In this study, we report the discovery and characterization of a new psychrophilic laccase, a multicopper oxidase (MCO), from the bacterium Oenococcus oeni. Laccases (benzenediol:oxygen oxidoreductase, p-diphenol oxidase EC 1.10.3.2) are blue multicopper oxidases (MCO), copper-containing enzymes that catalyse the oxidation of a substrate reducing molecular oxygen to water. Biochemical characterization of the psychrophilic laccase revealed its optimal activity at low temperatures, with a peak at 10 °C. To our knowledge, this is the lowest optimum temperature described so far for laccases. The structure of LcOe 229 showed the three specific structural features observed in the LAB laccases.

We obtained two types of crystals for LcOe 229, one for the enzyme without Histag and the other for the enzyme with Histag, that were grown under two different conditions and which diffracted X-rays to 3 and 3.5 Å, respectively, each one having a different monoclinic space group. Crystallization of LcOe 229 was achieved by mixing 0.3 µL of a solution containing 13 mg/mL of protein and 50 µM of CuCl2 with 0.2 µL of the same screening solutions. Crystals were grown in a condition containing 18% PEG 10000, 20% glycerol, 100 mM Tris-HCl pH 8.5, and 100 mM NaCl. Crystals were harvested and frozen directly as this condition also serves as cryoprotectant, then, they diffracted X-rays to 3 Å. For LcOe 229, the Ramachandran plot showed 93.7% residues in favoured regions, 6.21% in allowed regions, and 0.21% of outliers. The asymmetric unit of each crystal contained two molecules, which exploited two packing interfaces; however, according to the PISA server, both interfaces were the result of crystal packing. A comparison of the two molecules in the asymmetric unit of each crystal indicated that they were identical, even between both crystal types (RMSD between molecules was 0.2 Å for 476 residues), demonstrating absence of conformational changes between them. Interestingly, in both crystals of LcOe 229, we just could trace the C-terminal end until residue C477, which was forming a disulphide bond with residue C151 of Domain 1. There was no electron density for the last eleven residues, an indication of disorder and flexibility. The structure of LcOe 229 showed the T1Cu site with a Cu2+ ion coordinated by two His (H451 and H392), one Cys (C446), and one Met (M456).

>[2x]MELIKNYFFDEGAYDYHDGAYKHLIRPKTKMHKLIIPKVLKADKIEGNTTYYTIHAQEGETNILDGKATHTWGYNGSLLGPLIRYQSGRHYHLTLVNDLPEVTTWHWHGLNIPGPIEDGGPHAPVLPGKSREIKFDVNQPTMTAWLHPHPCPHTAEQVWKGLAAPVAVVNPLDDLPQLPHTWGVDDIPLIFQDRTFHDSQWDYQADYDMDGTLGDTALVNGTVNAEFTVTRPCLRLRVLNGANRRELRLNSDQNIVMTQIASDGGFLPHAIEMTKIMLTNAERAEILLDFSDYKKGDRIVLKADDVPILTLKVGEFTEDNRRQLPKTLKQIERDFTGSPSHQVIMEGMDDSVRINGKLYDMTRIDDRQEIGKNEIWDVSNTNDSMPGMGMIHPLHMHGTEFLVLSRNGKKPYPNEFGFKDTVAVNPGEHVKLLVKFNVPGIFMYHCHILEHEDTGMMAQIEAVDPNNPQHWNLKDLCDKNMPDSNMRM> MVFLPLKWSLATMSFLLSSLLALLTVSTPSWCQSTEASPKRSDGTPFPWNKIRLPEYVIPVHYDLLIHANLTTLTFWGTTKVEITASQPTSTIILHSHHLQISRATLRKGAGERLSEEPLQVLEHPRQEQIALLAPEPLLVGLPYTVVIHYAGNLSETFHGFYKSTYRTKEGELRILASTQFEPTAARMAFPCFDEPAFKASFSIKIRREPRHLAISNMPLVKSVTVAEGLIEDHFDVTVKMSTYLVAFIISDFESVSKITKSGVKVSVYAVPDKINQADYALDAAVTLLEFYEDYFSIPYPLPKQDLAAIPDFQSGAMENWGLTTYRESALLFDAEKSSASSKLGITMTVAHELAHQWFGNLVTMEWWNDLWLNEGFAKFMEFVSVSVTHPELKVGDYFFGKCFDAMEVDALNSSHPV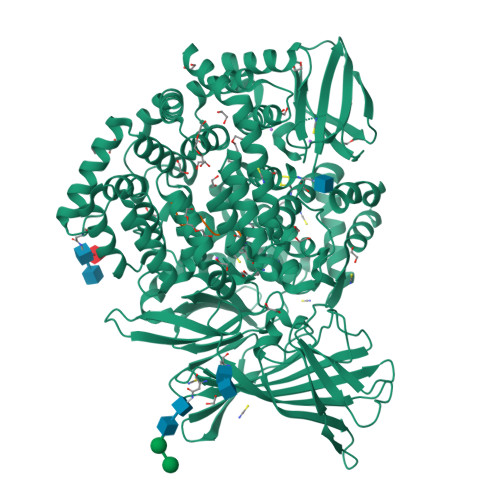STPVENPAQIREMFDDVSYDKGACILNMLREYLSADAFKSGIVQYLQKHSYKNTKNEDLWDSMASICPTDGVKGMDGFCSRSQHSSSSSHWHQEGVDVKTMMNTWTLQKGFPLITITVRGRNVHMKQEHYMKGSDGAPDTGYLWHVPLTFITSKSDMVHRFLLKTKTDVLILPEEVEWIKFNVGMNGYYIVHYEDDGWDSLTGLLKGTHTAVSSNDRASLINNAFQLVSIGKLSIEKALDLSLYLKHETEIMPVFQGLNELIPMYKLMEKRDMNEVETQFKAFLIRLLRDLIDKQTWTDEGSVSERMLRSQLLLLACVHNYQPCVQRAEGYFRKWKESNGNLSLPVDVTLAVFAVGAQSTEGWDFLYSKYQFSLSSTEKSQIEFALCRTQNKEKLQWLLDESFKGDKIKTQEFPQILTLIGRNPVGYPLAWQFLRKNWNKLVQKFELGSSSIAHMVMGTTNQFSTRTRLEEVKGFFSSLKENGSQLRCVQQTIETIEENIGWMDKNFDKIRVWLQSEKL;> XKHHAFSFK> GGTGGGGCTCGCCCCACC

Nine new crystal structures of CG-rich DNA 18-mers with the sequence 5′-GGTGGGGGC-XZ-GCCCCACC-3′, which are related to the bacterial repetitive extragenic palindromes, are reported. All 18-mers crystallized as isomorphic tetragonal crystals with one strand of a right-handed antiparallel duplex in the asymmetric unit. All reported structures co-crystallized with the Sr2+ cation located between nucleotides 6 and 7 and (by symmetry) 12 and 13.

NtC classes provided valuable help with building the initial models of six of the nine 18-mers, i.e. Chom-18-AT, Chom-18-CG, Chom-18-GC, Chom-18-GT, Chom-18-TC and Chom-18-AG. Although the number of unassigned steps remained the same in the Chom-18-TC structure, the average confal score and the average RSCC improved. The r.m.s.d.s between the NtC-restrained and nonrestrained models were 0.45 and 0.57 Å for the Chom-18-TC and Chom-18-CG structures, respectively. Of the four YY 18-mers, only Chom-18-CT could not be crystallized. Both Chom-18-TC and Chom-18-CC have high propeller twist; its extreme value in Chom-18-CC precludes assignment of the base-pair category. When we measure the distances between the C1′ atom of nucleotide 9 and C1′ of its symmetry-related base-paired nucleotide 10 in all 18-mers, the order from the shortest to the longest is TT (7.9 Å) < CC < TC < GT < GC < AC < AT < TA < CG < AG (12.1 Å). This trend follows the size of the pyrimidine–pyrimidine (Y–Y), pyrimidine–purine (Y–R/R–Y) and purine–purine (R–R) pairs regardless of the type of base pair involved.> MKAIAVKRGEDRPVVIEKPRPEPESGEALVRTLRVGVCGTDHEVIAGGHGGFPEGEDHLVLGHEAVGVVVDPNDTELEEGDIVVPTVRRPPASGTNEYFERDQPDMAPDGMYFERGIVGAHGYMSEFFTSPEKYLVRIPRSQAELGFLIEPISITEKALEHAYASRSAFDWDPSSAFVLGNGSLGLLTLAMLKVDDKGYENLYCLGRRDRPDPTIDIIEELDATYVDSRQTPVEDVPDVYEQMDFIYEATGFPKHAIQSVQALAPNGVGALLGVPSDWAFEVDAGAFHREMVLHNKALVGSV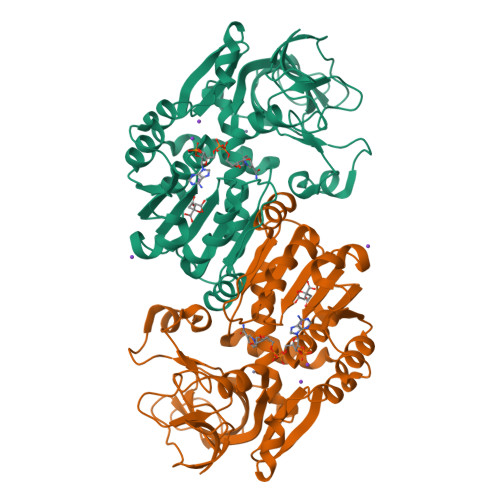NSHVEHFEAATVTFTKLPKWFLEDLVTGVHPLSEFEAAFDDDDTTIKTAIEFSTV>[2x]GPAGAQDDVPPYFKTEPVRTQVHLEGNRLVLTCMAEGSWPLEFKWLHNNRELTRFSLEYRYMITSLDRTHAGFYRCIVRNRMGALLQRQTEVQVAYMGSFEEGEKRQSVNHGEAAVIRAPRISSFPRPQVTWFRDGRKIPPSSRIAITLENTLVILSTVAPDAGRYYVQAVNDKNGDNKTSQPITLAVENVGGPADPIAPTIIIPPKNTSVVAGTSEVTMECVANARPLIKLHIVWKKDGAPLSSGISDYNRRLTIANPTVSDAGYYECEAMLRSSSVAPVTRGAYLSVLEPPQFVREPERHITAEMEKVVDIPCRAKGVPPPSITWYKDAALVEVGKLTRFKQRSDGGLQISGLLPDDTGMLQCFAHNAAGEAQTSTYLAVTS

Sdk1 and Sdk2 are single-pass transmembrane proteins, with extracellular regions composed of 6 N-terminal immunoglobulin (Ig) domains followed by 13 fibronectin type III (FNIII) domains, and a relatively short intracellular domain terminating in a Postsynaptic density/Discs Large/ZO-1 (PDZ) binding motif. Here, we report the crystal structures of cell-cell adhesive homophilic dimers of mouse Sdk1 and Sdk2, each mediated by the four N-terminal Ig domains. These four domains adopt a horseshoe conformation, like many other IgSF cell-cell recognition proteins, but they interact in a unique back-to-back anti-parallel manner not previously observed. Overall, our data suggest a model in which Sdks form cis dimers on isolated cell surfaces, which dissociate to form trans dimers through the same interface when contact is made to a cell surface expressing the cognate Sdk.

Two crystal forms of Sdk1Ig1–4 were determined at 2.2 and 3.2 Å resolution respectively, one of Sdk1Ig1–5 at 3.5 Å, two of Sdk2Ig1–4 at 2.7 and 3.2 Å respectively, and one of the Sdk2Ig1–2/Sdk1Ig3–4 chimera at 2.7 Å resolution. The second panel shows protomers from the two Sdk2Ig1–4 crystal forms structurally aligned, and the third panel shows a single protomer from the Sdk2Ig1–2/ Sdk1Ig3–4 structure. The dimer protomers are related by crystallographic 2-fold symmetry in both of the Sdk1Ig1–4 structures, and by non-crystallographic symmetry in all the other structures. Although the Ig1–2:Ig1–2 interaction is present in all of the crystal forms of Sdk1 and Sdk2, there is a difference in rotational angle between the two horseshoes of the dimer among the crystal forms, with the Ig1–2:Ig1–2 interface acting as the hinge. This results in differing levels of interaction between the Ig3–4 regions in the Sdk1 and Sdk2 dimers in the different crystal forms. The Ig3–4:Ig3–4 interaction varies from the Ig3–4 domains forming a considerable additional interface—as in Sdk1Ig1–4 crystal form 2 (915 Å2 BSA) and Sdk2Ig1–4 crystal form 1 (1294 Å2 BSA)—to being splayed 14 Å apart, as in the Sdk1Ig1–4 crystal form 1 structure (0 Å2 BSA). These differences indicate that there is flexibility in the interaction between the horseshoes in solution, with different conformations being trapped in the crystals. In addition to these major interfacial regions, the Sdk1Ig1–4 crystal form 2 also shows a small contact region between Ig1 residues E11 and R83 and Ig3 residue E212 towards the center of the horseshoe dimer. This interaction is not seen in either of the Sdk2 structures, although the residues are conserved.> MNARSTGQHPARYPGAAAGEPTLDSWQEPPHNRWAFAHLGEMVPSAAVSRRPVNAPGHALARLGAIAAQLPDLEQRLEQTYTDAFLVLRGTEVVAEYYR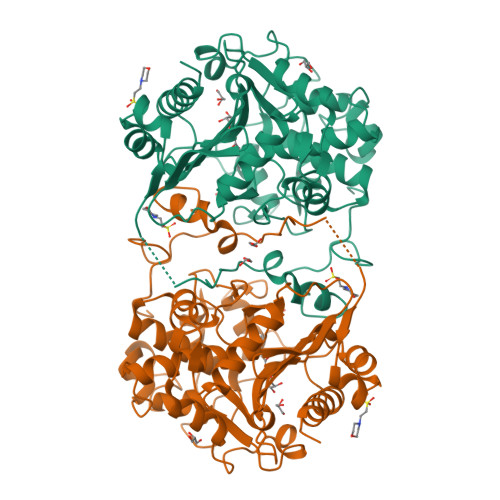AGFAPDDRHLLMAVSKSLCGTVVGALVDEGRIDPAQPVTEYVPELAGSVYDGPSVLQVLDMQISIDYNEDYVDPASEVQTHDRSAGWSTRRHGDPADTYEFLTTLRGDGSTGEFQYCSANTDVLAWIVERVTGLRYVEALSTYLWAKLDADRDATITVDTTGFGFANGGVSCTARDLARVGRMMLDGGVAPGGRVVSEDWVRRVLAGGSHEAMTDKGFTNTFPDGSYTRQWWCTGNERGNVSGIGIHGQNLWLDPLTDSVIVKLSSWPDPYTEHWHRLQNGILLDVSRALDAV>MSLPMLQVALDNQTMDSAYETTRLIAEEVDIIEVGTILCVGEGVRAVRDLKALYPHKIVLADAKIADAGKILSRMCFEANADWVTVICCADINTAKGALDVAKEFNGDVQIELTGYWTWEQAQQWRDAGIGQVVYARSRDAQAAGVAWGEADITAIKRLSDMGFKVTVTGGLALEDLPLFKGIPIHVFIAGRSIRDAASPVEAAR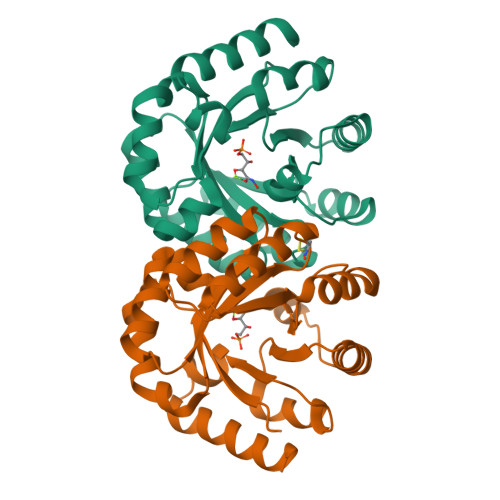QFKRSIAELWG[2x]> MEAGITGTWYNQLGSTFIVTAGADGALTGTYACGRGNAECRYVLTGRYDSAPATDGSGTALGWTVAWKNNYRNAHSATTWSGQYVGGAEARINTQWLLTSGTTEANAWKSTLVGHDTFTKVKPSAAS;> XS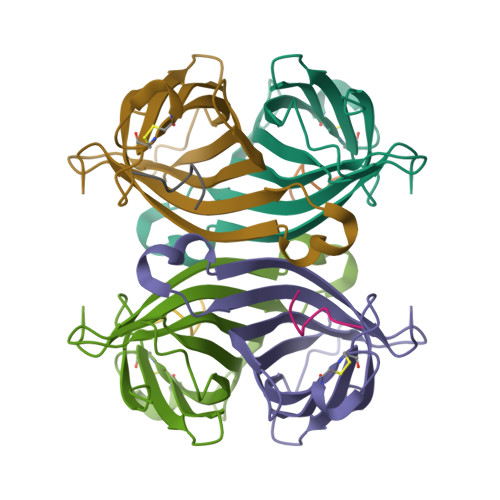AWSHPQFEKX>QECSLQSCTQHQPYVVDDPCPIHFYSKWYIRVGARKSAPLIELCVDEAGSKSPIQYIDIGNYTVSCLPFTINCQEPKLGSLVVRCSFYEDFLEYHDVRVVLDFI[2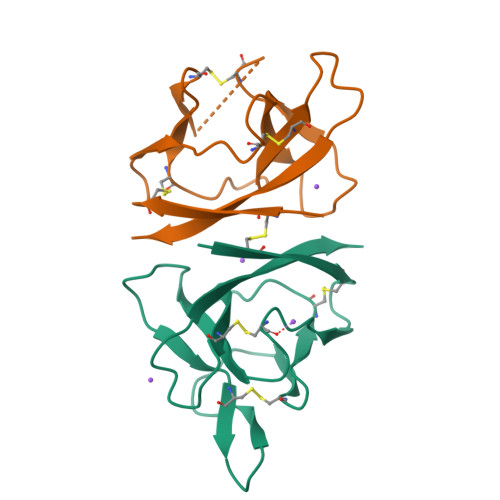x]> MKEVNVRESSQEREQRIQQQWQKGNVFQQSVQNREGYPSFVFYEGPPTANGLPGVHHALGRTIKDVVARYKTMTGHQVIRKAGWDTHGLPVELGVEKQLGISGKHDIEAYGVEAFINKCKESVFVYEKQWRTFTEQLGYWVDMEDPYITLENSYIESVWNVLGTIHDKGLLYKGHRVSPYCPSCQTSLSSHEVAQGYKDVKDLTVTVKFKVKNRDNEYFLGWTTTPWTLPSNVALAVHEEMSYVRAEQGDSVYIVAEALADKVLKGEYSVLSHHKGNELKGMSYEPPFNFVKVEKGHEVVTADYVTDQSGTGVVHLAPAYGEDDYRVVKENGFSFVNVVDEKGQYTSEVPPFQGRFVKDCDVDIVRYLANQDVLYHKEKHEHSYPFCWRCDSPLLYYANESWFIQTTALKEQFLKNNESVKWYPDHIKHGRFGKFLENMVDWNISRKRYWGTPLNVWECEGCQHQVAPKSIKELQKHASHYVDDSIELHKPYVDDVQLTCPVCSGEMKRTPEVIDVWFDSGSMPFAQYHYPFENSELFQKQFPADVIAEGIDQTRGWFYSLMAVSTLFTGKAPYKRVLSLGHVLDENGQKMSKSKGNALDPVDLIHTFGADALRWALLADSAPWNPKKFSERVVQEAKSKVIDTLVNVYGFYVLYAKLDGYDPEQTYELKKTKLDEWILSRLHSTVKRATVHLEDYGFTSAAREIAVFIEELSNWYVRRSRDRFWSEGMDGEKAAAYDTLHEVLVTLSQLLAPFTPFVADDVHENLTGKSVHLADYPACDQTKVNEKLEKEMAAVLQVVELGRSIRNTHSLKVKQPLQSLSLVVTEEDVEWKAYRDVIKDELNVKNFNVEQDDDKLVSYVLKLDFKQAGPKFGKQVNEVNQALKNLSEEKGKEFVEQGKLSVTLASGENLTLETEDVLVEKVPKEGFAVASNGMYTAVLDTALTEELVQEGVAREVIRAVQDYRKKLDLPVNSRINLELSGDEEVQKAVAKFETLLQENLLLHSLSVKETIKNGETVKVGTKQVVLRVLNQS

Mupirocin, a clinically used natural antibiotic, inhibits isoleucyl-tRNA synthetase (IleRS), an enzyme that links isoleucine to its tRNAIle for protein synthesis. Two IleRSs, mupirocin-sensitive IleRS1 and resistant IleRS2, coexist in bacteria. Specifically, type 1 proteins (IleRS1) are strongly inhibited by mupirocin (Ki in low nanomolar range), while IleRS2, which are homologous to IleRSs from the eukaryote cytosol, exhibit resistance to mupirocin concentrations that are about three orders of magnitude higher. AARSs catalyze the formation of AA-tRNA in two steps within the same active site. The amino acid is first activated by ATP to form an aminoacyl-adenylate (AA-AMP) intermediate, followed by the transfer of the aminoacyl moiety to the tRNA.

We mimic the motif alteration by the exchange of the first and third motif positions in PmIleRS2 that naturally carries the canonical HVGH motif. At the level of the overall fold, the WT enzymes and corresponding GXHH mutants are highly superimposable. The insights into why IleRS2, but not IleRS1, can tolerate the non-canonical signature motif came from the crystal structures of the pair of PmIleRS1 and PmIleRS2, both in complex with Ile-AMS. Specifically, in PmIleRS2, both wild-type and the GXHH-mutant, the tip of the helix α1 carrying the HXGH or GXHH motif is rearranged (shifted) and the α-carbon of the third motif residue is displaced (away from the adenosine) by 1.7 Å relative to the analogous position in PmIleRS1. To address this hypothesis, we in silico exchanged the canonical motif in the structure of wt-HVGH-PmIleRS2 bound to mupirocin with the GVHH sequence. The coordinates for the latter were taken from the mut-GVHH-PmIleRS2:Ile-AMS structure.> MSIQVTGIIEGPLGTPSPGITIRVVSKISYRNTYRLSTEDYVTTTGGAYDFQLNEGFHKILIRYRGASSFTKLGDVSVSDQTPSPITLINLLESSSPKALVVKLQELADEASESAQSASDDADQVTLDKQQVTLLAQQVSDDADQVALDRSATAQSEVNAAQSATTAQQSADDAAAIVPNLQSQIDDKIDKTQSIIPDVDALFSLGRHEINPTNNNIPGLSGTRSLLHIQNNLGGFQLAARTVGSEIHVRSADTNSGNIGPWERLYTTGYRPSSYDLVVKDKAEALSVSHQEGLIIGIESCNGARFVSVLPSDSGGLYLGSLPNGNKLRHIPLDGFSLKTIRTSDFEINSGSDVSQFLIDASTAGYGQVYIDNDC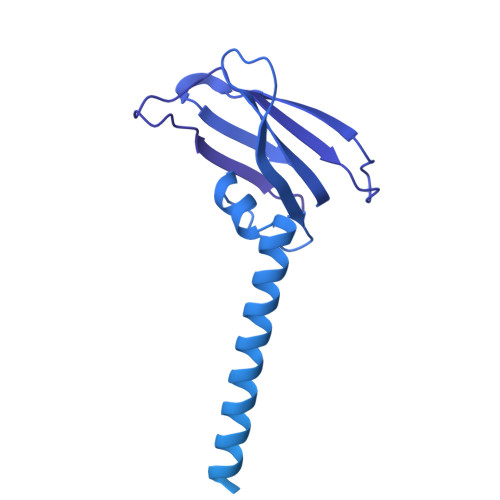EVTQLCDITGVKYLESLNGAEMLIDDLNGRVKCDTDGFEVKGIVFKKSGDYSNTTFEAYLLETNGEKSLASRCQFVGQWAGYKLQGNDSSADLCFFSDGTFMLRVGEGVSSCNINRCFFTRGTRRFTEGEQQGDGIKLTAQSSTQGYNENIIISDCIFYDTYRDCIDGYVGANRLIVKGSIMLNWGAHALDFKSRVDDNSESPDGGPLTRNVLVDGCMIWKDVVRPDFDLTLAAVVMSVIPGALPVPTSEADVRQNGLRGMELKNTLIAYKGNGSLISAASTWRTVIDGCTLTDLGQIGQIIYAPNSWHLKLINSTVNIDPSNINNVKFSSAMNNAEVNDNTFNRLLISTDGMIRTSIKRNKFNGEGVLSRGLNIASEEVSAVSNEFENFTSFGAQIFNSASKCRFDFNEIRNCPAPLGIENPSVNTYHSVRGNISMGSGAFTGLNRITDNGGVANGNDHVPYS beta-D-mannopyranuronic acid | C6 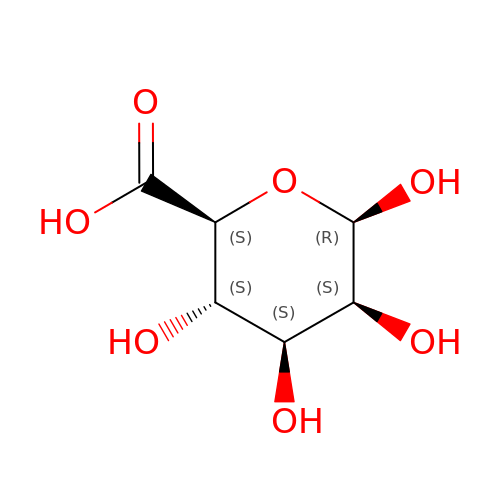H10 O7 | AEMOLEFTQBMNLQ-SYJWYVCOSA-N> QGGGRMRKKLYNDFAWECLRRNPQYISDWELFMKNTLTNGGGIPDDSELIQSELDLNAEKKWGVMKYIDPYNSDPTNVFWSLKLSNRSVRVKLSNTGNVKGGYTWGDMSNLPGVKHQRLLMHDNTLCVKIFSQNGYFQLFIESADALKDXXXXXXXXXXXXXXXXXXXXXXXXXXIVNHKIEVECKEEQYLGLLKTIDDRKQGFSHRDIASEIFGKELVKNEWSADSWVRAKIRYRIKKANALINYGYLNFL

The type VI secretion system (T6SS) is a complex, versatile multiprotein nanomachine, which is dedicated to the delivery of toxic effectors into prokaryotic and eukaryotic cells. RovC is a transcriptional regulator that strongly induces expression of the T6SS4 at moderate temperatures in stationary growth phase. It folds into a novel hexameric structure with surface-exposed DNA-binding sites, which directly interact with an extended sequence in the T6SS4 promoter region. Expression of the rovC gene is tightly regulated by the global nutrient-responsive regulator CsrA, and induction of its synthesis is essential for the transcriptional activation of the secretion system genes, independently of RovM.

To gain a better insight into the structure and function of this novel DNA-binding protein, we determined its crystal structure to 2.3 Å resolution. RovC consists of two distinct domains. The C-terminal domain (181–247, pink) is formed by five α-helices which fold into a helix-turn-helix motif, as predicted. The N-terminal domain comprises amino acids 1–136 (orange) and a central region (gray). Amino acids 1–136 fold into four α-helices and a mixed β-sheet with four β-strands. While a secondary structure can be assigned to the central region (gray) that forms an elongated stretch of amino acids, an unambiguous assignment of individual amino acids to this elongated stretch (gray) was not possible due to ill-defined electron density and flexible/unstructured loops which connect it to the rest of the protein. The asymmetric unit of crystallized RovC contains one molecule. However, extending the crystal lattice by generating the crystallographic symmetry-related RovC molecules reveals a hexameric ring-shaped structure composed of three RovC dimers (interface between monomers: interface I) in which the interface between the dimers (interface II) is formed solely by the N-terminal domain. One extended basic patch (formed by a RovC dimer) was identified on the outer surface of the ring mainly formed by residues 225–240 present on the helix-turn-helix motif which is likely to be involved in the interaction with the negatively charged DNA backbone. DNA binding assays further revealed that the R225E and R202E substitution completely abolished the DNA-binding activity of RovC, while the DNA-binding activity of the inducing K175E mutant remained unaffected.(2~{S})-3-(2-bromophenyl)-2-[2-(4-methoxyphenyl)ethanoylamino]-~{N}-[(1~{S})-1-phenylethyl]propanamide 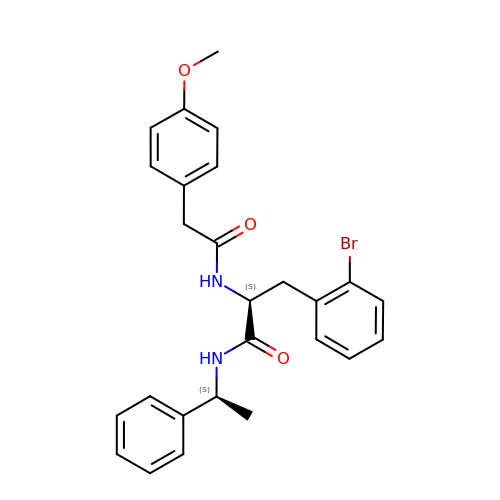| C26 H27 Br N2 O3 | ZFUNKFOMZPXBEZ-UUOWRZLLSA-N>MKDYKSITIATEGSYAPYNFKDAGGKLIGFDIDLGNDLCKRMNIECKFVEQAWDGIIPSLTAGRYDAIMAAMGIQPAREKVIAFSRPYLLTPNTFLTTADSPLLKTQVAIENLPLDNITPEQKAELDKFTKIFEGVKFGVQAGTSHEAFMKQMMPSVQISTYDTIDNVVMDLKAGRIDASLASVSFLKPLTDKPDNKDLKMFGPRMTGGLFGKGVGVGIRKEDADLKALFDKAIDAAIADGTVQKLSQQWFGYDASPKQHHHHHH[2x]

In A. tumefaciens, the recognition and import of opines is conferred by periplasmic binding proteins (PBPs) and their associated ATP-binding cassette (ABC) transporters; but there is no known structure of the opine-PBP complex. In this work, we investigated the structural and biochemical properties of the PBP NocT of A. tumefaciens C58 which senses at least two opines: nopaline and pyronopaline, a lactam nopaline-derivative that can also be found in plant tumours. NocT possesses a typical fold of cluster F within the PBP structural classification. The ligand-binding site of NocT was defined by the Glu36, Tyr39, Tyr42, Trp77, Ala94, Ala95, Gly97, Arg102, Thr115, Met117, Gln165, Thr168, Ser169, His170, Ser207, Gly238 and Val239 residues.

To learn more on the role of Met117 residue in the interaction between NocT and its ligand, we constructed two NocT mutants with different short polar residues: NocT-M117N because an asparagine is found in the OccJ sequence and NocT-M117S because a serine is found in the LAO/HisJ sequences. Both mutants displayed a similar KD for pyronopaline that was 76-fold higher than that of the WT protein, proving that Met117 is a key component of the ligand affinity and belongs to the nopaline-binding signature. We also obtained the structure of NocT-M117N in complex with pyronopaline. Prior to this, the stability of NocT-M117N was verified using differential scanning calorimetry (DSC) and, compared to the WT protein, the mutant presented similar Tm (60.12°C versus 60.25°C for the WT) and ΔH (1.59 105 cal/mol/°C versus 1.4 105 cal/mol/°C for the WT), meaning that mutating M117 has no significant effect on protein stability. The structure of NocT-M117N in complex with pyronopaline confirmed that the replacement of Met117 with Asn led to a loss of hydrophobic interaction with the ligand and showed that His170 which is free to move towards Asn117 bound the carboxyl group of the α-KG of the pyronopaline in a position not observed in the WT complexes. A loss of the polar interaction between the side chain of Ser169 and the terminal OH of the pyronopaline ring was also observed due to steric hindrance.N,N-dibutyl-4-chloranyl-1-[2-(3,4-dihydro-1H-isoquinolin-2-ylcarbonyl)-4-[(7-iodanylnaphthalen-2-yl)sulfonylcarbamoyl]phenyl]-5-methyl-pyrazole-3-carboxamide 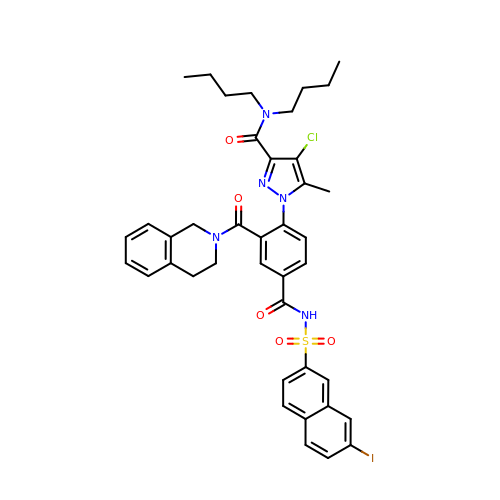| C40 H41 Cl I N5 O5 S | DKJBPPVETUSFTM-UHFFFAOYSA-N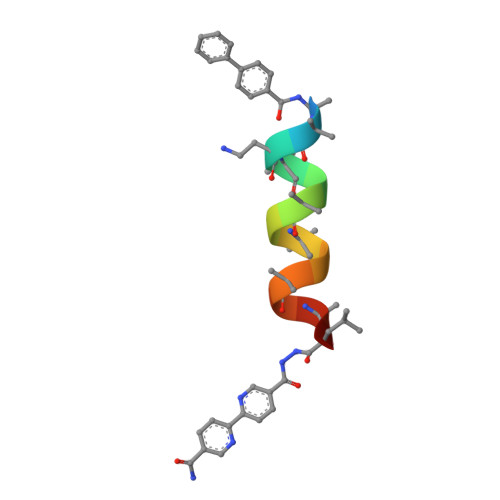>[4x]XAAAALAAALAQALX FLAVIN-ADENINE DINUCLEOTIDE-N5-ISOBUTYL KETONE | C31 H39 N9 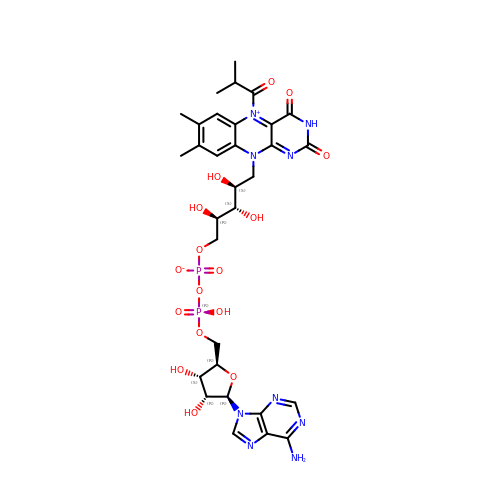O16 P2 | VVZGWZAMSAFRNS-UYOVOMPXSA-N Gaucher disease (GD) is the most common lysosomal storage disorder which is caused by inherited deficiencies in β‐glucocerebrosidase (glucosylceramidase, GCase, GBA, EC 3.2.1.45). GBA is primarily responsible for catalyzing the degradation of GlcCer by hydrolytic cleavage of the β‐glucose moiety from the aglycone to yield free ceramide and glucose. This is achieved with retention of β‐anomeric stereochemistry of the released glucose unit through a Koshland double displacement mechanism using Glu340 as the catalytic nucleophile and Glu235 as the catalytic acid‐base. Here, we report the design, synthesis, and structural analysis of a range of cyclophellitol epoxide and aziridine inactivators and activity‐based probes (ABPs) for human β‐glucocerebrosidase (GBA).

To further understand the binding of galacto‐configured cyclophellitol aziridines with rhGBA, a co‐crystal structure with galacto‐configured 4 was obtained at 1.80 Å. The resulting complex revealed that 4 covalently modifies the catalytic nucleophile of GBA in an almost identical fashion to gluco‐configured reagents 1 and 2. Specifically, 4 reacts with Glu340 via trans‐diaxial ring opening of the aziridine trap to form a covalent complex in the 4C1 conformation with a bond length of 1.45 Å. The key difference between this galacto‐configured complex and the gluco‐configured analogues is the axial conformation of the O4 hydroxyl, which is still able to form a hydrogen bond with Asp127. Indeed, the hydrogen bonding network of 4 is very similar to that of gluco‐configured 1 and 2, with both O3 and O4 able to form hydrogen bonds to Asp127 regardless of whether the sugar is gluco‐ or galacto‐configured. The only notable difference is the absence of a hydrogen bond between the O4 hydroxyl and Trp381, presumably owing to its axial conformation. Overlay of galacto‐aziridine 4 and gluco‐epoxide 1 provides an immediate clue: the O6 hydroxyl of galacto‐aziridine 4 has rotated such that it points ‘downwards’, perhaps to avoid steric clash with the axial galacto‐O4. Thus, one possible explanation for the cross‐reactivity of galacto‐aziridines but not O6‐substituted galacto‐epoxides, is the requirement to displace the O6‐hydroxyl for covalent binding which would not be possible were the O6‐substituted. Therefore, it appears that the placement of the reporter group is important in controlling the selectivity and cross‐reactivity of cyclophellitol‐based ABPs. In combination with the ABP labelling assays of rhGBA, this co‐crystal structure serves as a caution when assuming similar configurational specificity of cyclophellitol epoxides and aziridines, which evidently does not always translate to similar glycosidase specificity.

>ARPCIPKSFGYSSVVCVCNATYCDSFDPPTFPALGTFSRYESTRSGRRMELSMGPIQANHTGTGLLLTLQPEQKFQKVKGFGGAMTDAAALNILALSPPAQNLLLKSYFSEEGIGYNIIRVPMASCDFSIRTYTYADTPDDFQLHNFSLPEEDTKLKIPLIHRALQLAQRPVSLLASPWTSPTWLKTNGAVNGKGSLKGQPGDIYHQTWARYFVKFLDAYAEHKLQFWAVTAENEPSAGLLSGYPFQCLGFTPEHQRDFIARDLGPTLANSTHHNVRLLMLDDQRLLLPHWAKVVLTDPEAAKYVHGIAVHWYLDFLAPAKATLGETHRLFPNTMLFASEACVGSKFWEQSVRLGSWDRGMQYSHSIITNLLYHVVGWTDWNLALNPEGGPNWVRNFVDSPIIVDITKDTFYKQPMFYHLGHFSKFIPEGSQRVGLVASQKNDLDAVALMHPDGSAVVVVLNRSSKDVPLTIKDPAVGFLETISPGYSIHTYLWHRQ[2x]>[8x]GSEGQKKRRNTLHEFKKSAKTTLTKEDPLLKIKTKKVNSADEC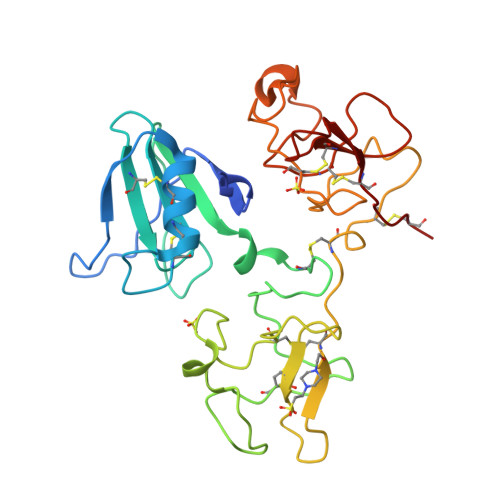ANRCIRNRGFTFTCKAFVFDKSRKRCYWYPFNSMSSGVKKGFGHEFDLYENKDYIRNCIIGKGGSYKGTVSITKSGIKCQPWNSMIPHEHSFLPSSYRGKDLQENYCRNPRGEEGGPWCFTSNPEVRYEVCDIPQCSEVECMTANGESYRGPMDHTESGKTCQRWDQQTPHRHKFLPERYPDKGFDDNYCRNPDGKPRPWCYTLDPDTPWEYCAIKTCA Here, we report heterologous expression and production of soluble biologically active FTP in E. coli and also describe the crystal structure of Apo-FTP plus changes on binding α-D-glucose or α-D-mannose. The FTP structure showed a β-prism I fold, which is found in Jacalin, Artocarpin and other lectins giving a high structural similarity; except for a few loop areas around residues Leu90, Glu36 and Lys106, some of which are flexible and adopt different conformations, even in the same protein. Like most-known plant lectins, FTP is a hololectin defined as a multisubunit protein containing several carbohydrate-binding sites to allow cell agglutination. In contrast, FTP binds carbohydrates such as mannose and/or glucose in a different way, paralleling CMB and also Artocarpin presumably reflecting the high sequence identities of 90 and 91%, respectively.

FTP was also co-crystallized with mannose and glucose; the crystals diffracted to a resolution of 1.70 and 1.60 Å respectively. Although these grew in similar conditions to the Apo-crystals, data processing revealed a different space group: P3121 rather than P212121. FTP–mannose crystals were twinned by merohedry with a twinning fraction of 22.4%. Both ligand structures showed clear electron density for their respective sugars in the carbohydrate-binding sites of all the four molecules in their asymmetric units, but did not present relevant structural differences when compared with Apo-FTP protein. The crystal structures of FTP–glucose and FTP–mannose complexes also show this feature: HBs occur between Gly16, Leu90, Gly138, Asp139, Leu140, Asp142 and O3, O4, O5, O6 of the carbohydrates, but they vary slightly both in number and strength from subunit to subunit. In the FTP–mannose structure, the sugar ring is in the energetically favourable boat conformation. By studying crystals of the FTP–mannose complex, a water molecule was found between mannose and Asp139 consistent with their lower interaction. In case of FTP–mannose, HBs were detected between Leu90 (C=O) and mannose (H–O1), an interaction not observed in FTP–glucose. Therefore, mannose is better surrounded in the carbohydrate-binding site and is also stabilized by indirect interaction with Asp139 through water molecules, which helps to stabilize the sugar in the binding site. This local structuring is more stable in the case of mannose than glucose indicating higher affinity of FTP for mannose than glucose.

>MASQTITVGPWGGPGGNEWDDGSYTGIRIIELSYKEAIGSFSVIYDLNGEPFSGSKHTSKLPYTNVKIELQFPEEFLVSVSGYTAPFSSLATRTPVVRSLKFKTNKGRTFGPYGEEDGTYFNLPIENGLVVGFKGRTGDLLDAIGVHMAL[4x]>PVVKINAIEVPAGAGPELEKRFAHSAHAVENSPGFLGFQLLRPVKGEERYFVVTHWESDEA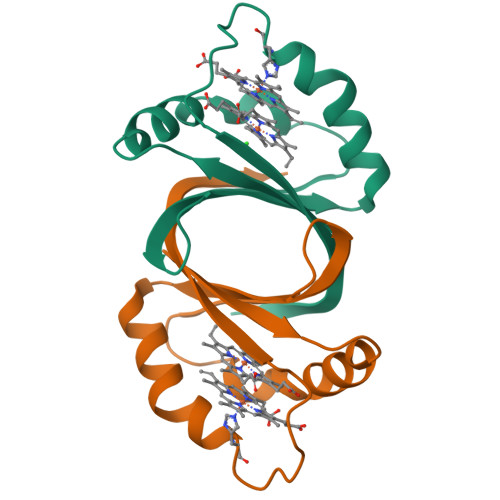FQAWANGPAIAAHAGHRANPVATGASLLEFEVVLDVGG[2x]> PQYQTWEEFSRAAEKLYLADPMKARVVLKYRHSDGNLCVKVTDDLVCLVYKTDQAQDVKKIEKFHSQLMRLMVAKE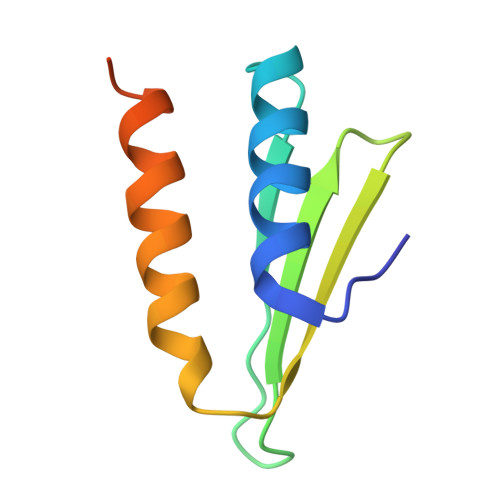ARNVTMETE> MNPMYVSKLSLVLVAAALVGACATKPAPDFGGRWKHVNHFDEAPTEIPLYTSYTYQATPMDGTLKTMLERWAADSNMQLSYNLPSDYTLIGPVSAIST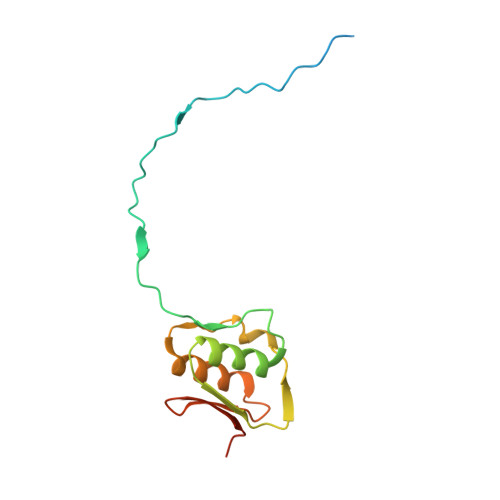TSVQQAATELSAVYAAQGVSVSVSANKLLVQPVPVSSGAKL>[4x]MSQRGLEALLRPKSIAVIGASMKPNRAGYLMMRNLLAGGFNGPVLPVTPAWKAVLGVLAWPDIASLPFTPDLAVLCTNASRNLALLEELGEKGCKTCIILSAPASQHEDLRACALRHNMRLLGPNSLGLLAPWQGLNASFSPVPIKRGKLA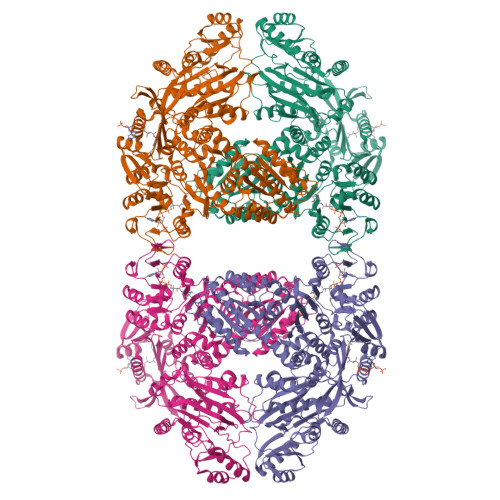FISQSAAVSNTILDWAQQRKMGFSYFIALGDSLDIDVDELLDYLARDSKTSAILLYLEQLSDARRFVSAARSASRNKPILVIKSGRSPAAQRLLNTTAGMDPAWDAAIQRAGLLRVQDTHELFSAVETLSHMRPLRGDRLMIISNGAAPAALALDALWSRNGKLATLSEETCQKLRDALPEHVAISNPLDLRDDASSEHYIKTLDILLHSQDFDALMVIHSPSAAAPATESAQVLIEAVKHHPRSKYVSLLTNWCGEHSSQEARRLFSEAGLPTYRTPEGTITAFMHMVEYRRNQKQLRETPALPSNLTSNTAEAHLLLQQAIAEGATSLDTHEVQPILQAYGMNTLPTWIASDSTEAVHIAEQIGYPVALKLRSPDIPHKSEVQGVMLYLRTANEVQQAANAIFDRVKMAWPQARVHGLLVQSMANRAGAQELRVVVEHDPVFGPLIMLGEGGVEWRPEDQAVVALPPLNMNLARYLVIQGIKSKKIRARSALRPLDVAGLSQLLVQVSNLIVDCPEIQRLDIHPLLASGSEFTALDVTLDISPFEGDNESRLAVRPYPHQLEEWVELKNGERCLFRPILPEDEPQLQQFISRVTKEDLYYRYFSEINEFTHEDLANMTQIDYDREMAFVAVRRIDQTEEILGVTRAISDPDNIDAEFAVLVRSDLKGLGLGRRLMEKLITYTRDHGLQRLNGITMPNNRGMVALARKLGFNVDIQLEEGIVGLTLNLAQREES>GSHMAPDSQVCDVGSTATCKITATPRQFQPALLSTSKWIWTGENPIPGGSNIISTRPFRKNITAPCGKCSVCATIVVASDDAHTFYVNGVRIGTGAGFRQGQALFVALQPTWNLFAIAGQNLVANSPAGIMASILVHFSDGTSETFVTDESWKTLRAAPPENFQLPSTNDSNWPSAAVQGAYQNSVWGPPVLPPVLPLRGSNWIWTSDNVNGAAPVGSRAFRKTVNQCTKVAVCATVLIAADDRYTLYVNGATVGSGSSYTV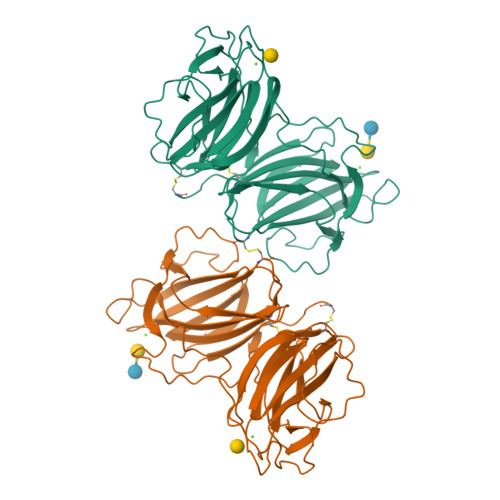ADAYTIPNLHPTFNTFAINATNGGGPAGVIATILITYSDGSNETVVTDASWKAIQTIPQGFQPPLIDEFGWESAKIIGAFGVAPWGAGMVIPSA[6x]pyrrolidin-2-one | C4 H7 N O | 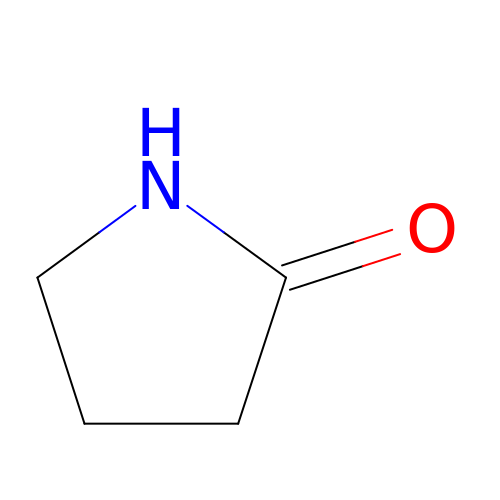HNJBEVLQSNELDL-UHFFFAOYSA-N> PPLPEHGGKVRLGLIPE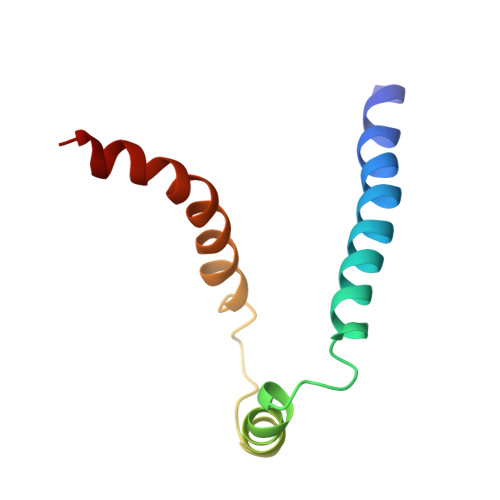EFFQFLYPKTGVTGPYVLGTGLILYLLSKEIYVITAETFSAISTIGVLVYIVKKYGASIGAFADK> MLNILKNWKNQQTAASNLERYTKEDILKGEIPEHIAIIMDGNGRWAKKRSLPRIAGHHEGMKVVKRTTKLANELGVKVLTLYAFSTENWKRPKMEVDFL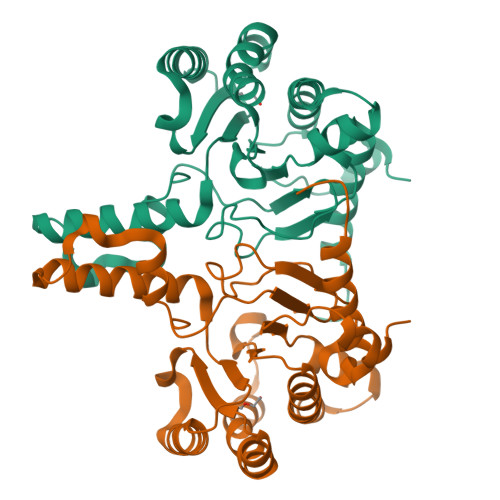MKLPEEFLNTYLPELVEENVQVRIIGDETALPAHTLRAIEKAVQDTAQNDGMILNFALNYGGRTEIVSAAKSLAEKVKEGSLNIEDIDESLFSTYLMTESLQDPELLIRTSGEIRLSNFMLWQVAYSEFVFTDVLWPDFKEDHFLQALGEFQQRGRRFGGI>[12x]MAHHHHHHVDDDDKTSGQIKVLYANKETNSTTNTIRPWLKVVNTGSSSIDLSRVTIRYWYTVDGDRAQSAISDWAQIGASNVTFKF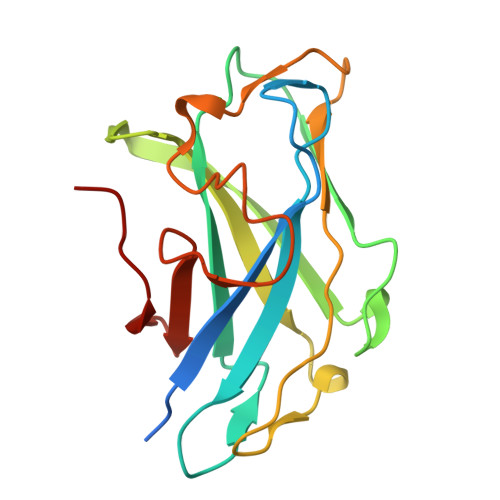VKLSSSVSGADYYLEIGFKSGAGQLQPGKDTGEIQIRFNKSDWSNYNQGNDWSWLQSMTSYGENVKVTAYIDGVLVWGQEPSGA> XLAASLAC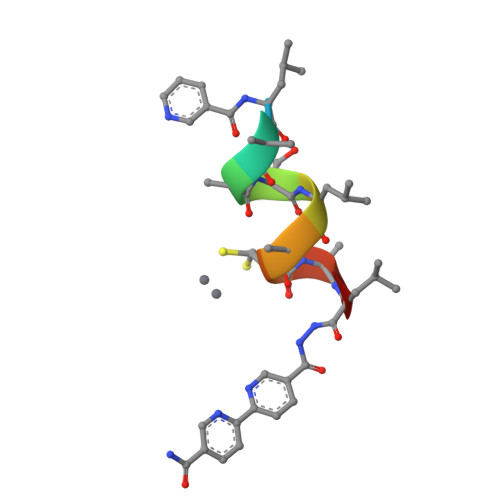ALX>[2x]MHHHHHHAMEEVTIKANLIFANGSTQTAEFKGTFEKATSEAYAYADT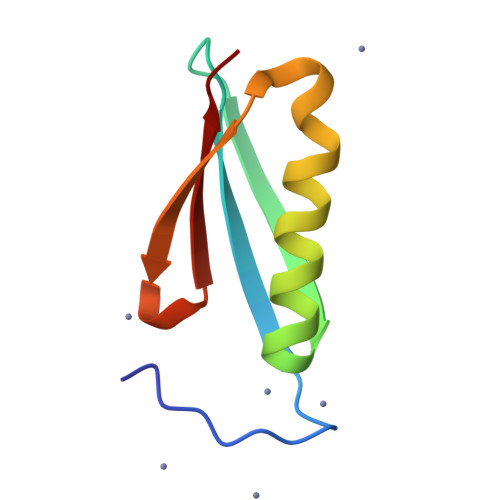LKKDNGEWTVDVADKGYTLNIKFAG>DWVIAAISCPENEKGEFPKNLVQIKSNRDKETKVFYSITGQGADKPPVGVFIIERETGWLKVTQPLDREAIAKYILYSHAVSSNGEAVEDPMEIVITVTDQNDNRPEFTQEVFEGSVAEGAVPGTSVMKVSATDADDDVNTYNAAIAYTIVSQDPELPHKNMFTVNRDTGVISVLTSGLDRESYPTYTLV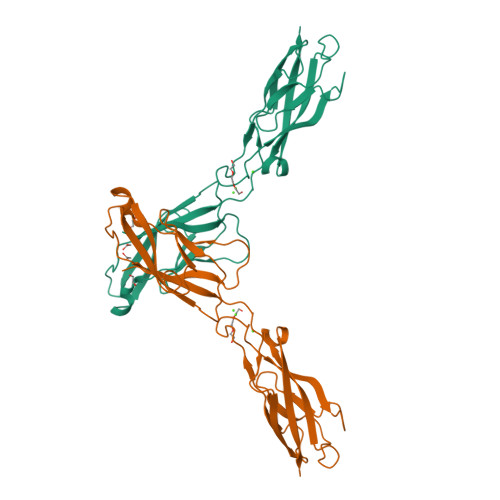VQAADLQGEGLSTTAKAVITVKD[2x]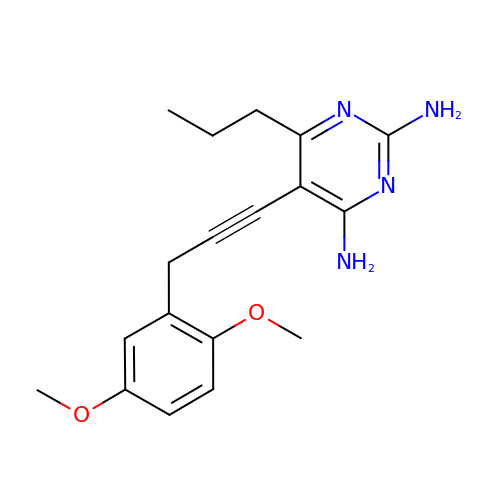5-[3-(2,5-dimethoxyphenyl)prop-1-yn-1-yl]-6-propylpyrimidine-2,4-diamine | C18 H22 N4 O2 | VSWSZIRWLYCVMG-UHFFFAOYSA-N> MSVVSQVILQADDQLRYPTSGELKGIQAFLTTGAQRIRIAETLAENEKKIVDQAQ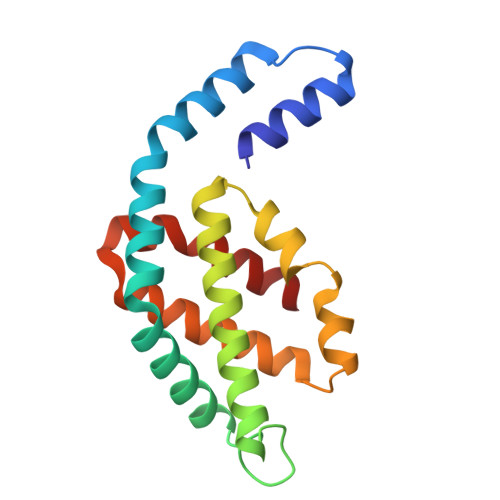KQLFKKHPEYRAPGGNAYGQRQYNQCLRDYGWYLRLVTYGVLAGNKEPIETTGLIGVKEMYNSLNVPVPGMVDAVTVLKDAALGLLSAEDANETAPYFDYIIQFMS> SNAMKKIHPSAVIEEGAQLGDDVVIEAYAYVSKDAKIGNNVVIKQGARILSDTTIGDHSRVFSYAIVGDIPQDISYKEEQKSGVVIGKNATIREFATINSGTAKGDGFTRIGDNAFIMAYCHIAHDCLLGNNIILANNATLAGHVELGDFTVVGGLTPIHQFVKVGEGCMIAGASALSQDIVPFCLAEGNRASIRSLNLVGIRRRFDKDEVDRLSRAFKTLFRQGDLK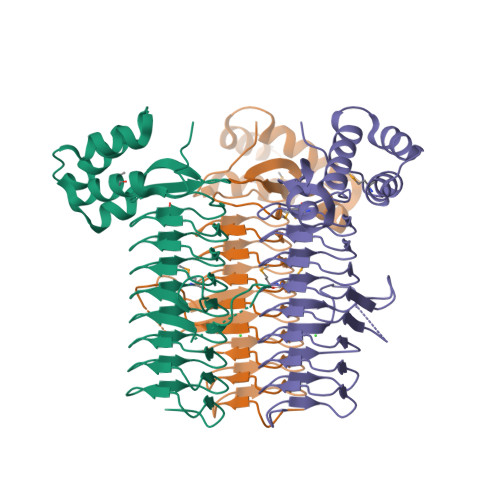ENAKNLLENQESENVKKMCHFILETKRGIPVYRGKNNA(2E)-3-[3-(3-ETHOXY-5,5,8,8-TETRAMETHYL-5,6,7,8-TETRAHYDRONAPHTHALEN-2-YL)-4-HYDROXYPHENYL]ACRYLIC ACID 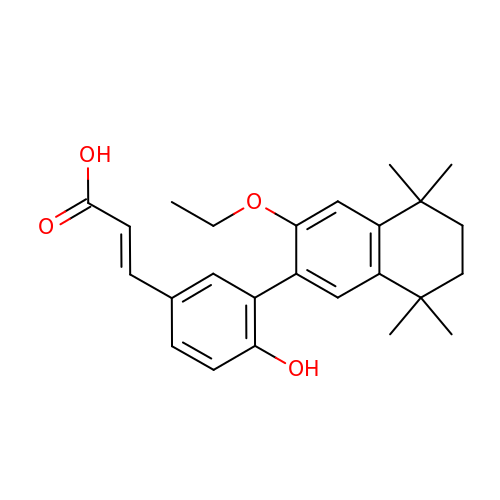| C25 H30 O4 | FXYICDGGLYXLPD-CSKARUKUSA-N>GAPEVSHVRGVTVRMETPEAILFSPGETFSTNVSIHAIAHDDQTYSMDVVWLRFDVPTSCAEMRIYESCLYHPQLPECLSPADAPCAASTWTSRLAVRSYAGCSRTNPPPRCSAEAHMEPVPGLAWQAAS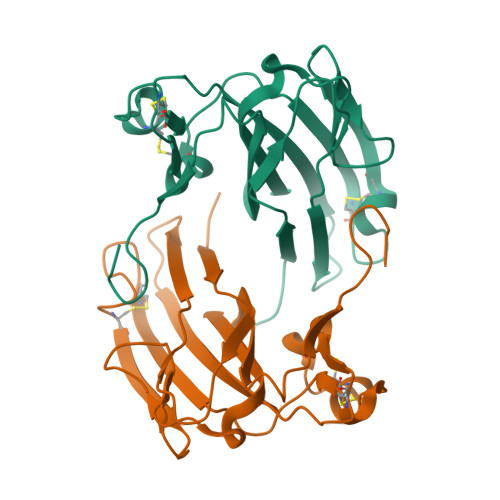VNLEFRDASPQHSGLYLCVVYVNDHIHAWGHITISTAAQYRNAVVEQPLDIEGRGHHHHHH[2x]>MKVALGGTFEPLHEGHKKLIDVAIKLGGRDITIGVTSDRMARARIRSVLPFAIRAENVKRYVMRKYGFEPEIVKITNPYGKTLDVDFEYLVVSPETYEMALKINQKREELGKRKITIVKVDWMMAEDGKPISSTRIKRGEID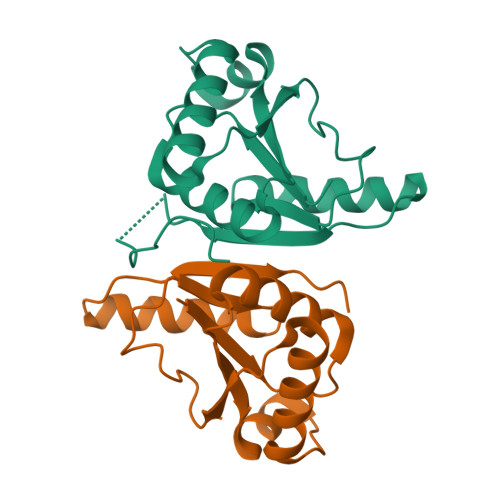RYGGII[2x]>[2x]SHMKFTVEREHLLKPLQQVSGPLGGRP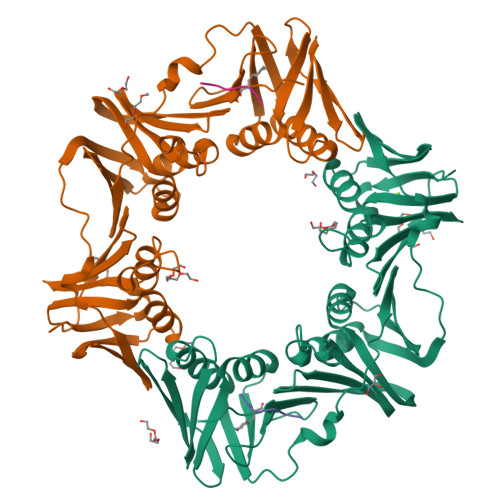TLPILGNLLLQVADGTLSLTGTDLEMEMVARVALVQPHEPGATTVPARKFFDICRGLPEGAEIAVQLEGERMLVRSGRSRFSLSTLPAADFPNLDDWQSEVEFTLPQATMKRLIEATQFSMAHQDVRYYLNGMLFETEGEELRTVATDGHRLAVCSMPIGQSLPSHSVIVPRKGVIELMRMLDGGDNPLRVQIGSNNIRAHVGDFIFTSKLVDGRFPDYRRVLPKNPDKHLEAGCDLLKQAFARAAILSNEKFRGVRLYVSENQLKITANNPEQEEAEEILDVTYSGAEMEIGFNVSYVLDVLNALKCENVRMMLTDSVSPVQIEDAASQSAAYVVMPMRL;>[2x]XQADLF> MSGMLDELFSLLNKMFELSDKYRELRKELRKAIESGAPEEELRELLEKMLEIAKKLLELTKELKKLVEDVLKNNPDPVERAKAVLLYAVGVHILYSESSELEVIAERLGFKDIAEKAKEIADKARELKEEVKRKLREIREEVPDPEIRKAAEEAIEMLESNDKRLKEFRKLHSQ;> GFTSDYSKYLDSRRAQDFVQWLMNT

Peptide hormones, such as parathyroid hormone (PTH), neuropeptide Y (NPY), glucagon (GCG) and secretin (SCT), which adopt α-helical structures on binding their receptors, play key roles in human biology and are well-established biomarkers in clinical care and biomedical research. We set out to develop general methods for designing proteins that bind peptides in helical conformations. We show that by extending RFdiffusion8 to enable binder design to flexible targets, and to refining input structure models by successive noising and denoising (partial diffusion), picomolar-affinity binders can be generated to helical peptide targets by either refining designs generated with other methods, or completely de novo starting from random noise distributions without any subsequent experimental optimization. The deep learning methods largely converged on the overall solution to the helical peptide-binding design problem—groove-shaped scaffolds with helices lining the binding site—that the human designers chose in the initial Rosetta parametric approaches.

We used the same design strategy to generate higher-affinity binders for NPY and GCG. Using weak parametric binders as a starting point, we extended their binding interfaces and redesigned their sequences to generate a 231-nM-affinity binder for GCG and a 3.5-µM binder for NPY after screening 96 designs. As a first experimental test of partial diffusion, we started from our parametrically designed Inpainted binders to GCG (with 231 nM Kd) and NPY (with 3.5 µM affinity). To gain insight into the structural rearrangements generated by partial diffusion that contribute to the affinity increases, we solved the structures of the original Inpainted GCG binder and the partially diffused higher-affinity GCG binder. Both designs were very close to their design models. Alignment of the two crystal structures on the structurally conserved C-terminal residues (16–29) of GCG showed that in the partially diffused GCG binder a 2.7-Å shift towards the target in the binder backbone enables an isoleucine to fit into a pocket previously occupied by a phenylalanine side chain at position 13 (left inset). Similarly, at position 16, a 3.6-Å shift in the backbone allows a tyrosine residue to pack underneath the peptide and form a hydrogen bond to the peptide backbone where previously a serine could not make any contacts (right inset). These backbone movements and accompanying sequence changes increase the interaction shape complementarity (0.62 versus 0.67) and contact molecular surface (431 Å2 versus 522 Å2; computed on the crystal structures).>ADKLFINALKKKFEESPEEKKTTFYTLGGWKQSERKTEFVNAGKEVAAKRGIPQYNPDIGTPLGQRVLMPYQVSTTDTYVEGDDLHFVNNAAMQQMWDDIRRTVIVGLNHAHAVIEKRLGKEVTPETITHYLETVNHAMPGAAVVQEHMVETHPALVADSYVKVFTGNDEIADEIDPAFVIDINKQFPEDQAETLKAEVGDGIWQVVRIPTIVSRTCDGATTSRWSAMQIGMSMISAYKQAAGEAATGDFAYAAKHAEVIHMGTYLPVRRARGENEPGGVPFGYLADICQSSRVNYEDPVRVSLDVVATGAMLYDQIWLGSYMSGGVGFTQYATAAYTDNILDDFTYFGKEYVEDKYGLCEAPNNMDTVLDVATEVTFYGLEQYEEYPALLEDQFGGSQRAAVVAAAAGCSTAFATGNAQTGLSGWYLSMYLHKEQHSRLGFYGYDLQDQCGASNVFSIRGDEGLPLELRGPNYPNYAMNVGHQGEYAGISQAPHAARGDAFVFNPLVKIAFADDNLVFDFTNVRGEFAKGALREFEPAGERALITPAK[2x];>[2x]AKFEDKVDLYDDRGNLVEEQVPLEALSPLRNPAIKSIVQGIKRTVAVNLEGIENALKTAKVGGPACKIMGRELDLDI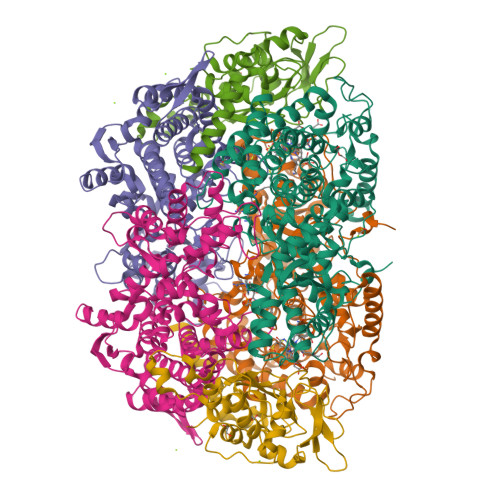VGNAESIAAAAKEMIQVTEDDDTNVELLGGGKRALVQVPSARFDVAAEYSAAPLVTATAFVQAIINEFDVSMYDANMVKAAVLGRYPQSVEYMGANIATMLDIPQKLEGPGYALRNIMVNHVVAATLKNTLQAAALSTILEQTAMFEMGDAVGAFERMHLLGLAYQGMNADNLVFDLVKANGKEGTVGSVIADLVERALEDGVIKVEKELTDYKVYGTDDLAMWNAYAAAGLMAATMVNQGAARAAQGVSSTLLYYNDLIEFETGLPSVDFGKVEGTAVGFSFFSHSIYGGGGPGIFNGNHIVTRHSKGFAIPCVAAAMALDAGTQMFSPEATSGLIKEVFSQVDEFREPLKYVVEAAAEIKNEI;>[2x]AQYYPGTTKVAQNRRNFCNPEYELEKLREISDEDVVKILGHRAPGEEYPSVHPPLEEMDEPEDAIREMVEPIDGAKAGDRVRYIQFTDSMYFAPAQPYVRSRAYLCRYRGADAGTLSGRQIIETRERDLEKISKELLETEFFDPARSGVRGKSVHGHSLRLDEDGMMFDMLRRQIYNKDTGRVEMVKNQIGDELDEPVDLGEPLDEETLMEKTTIYRVDGEAYRDDVEAVEIMQRIHVLRSQGGFNLE>[4x]MASLARAVERLKAALERPKDEFI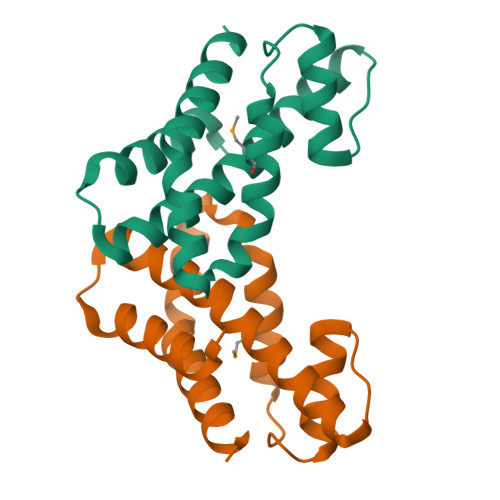RDSAIQRFEFTFELAWKTLKTFLELQGLEARSPRAAIRGAFQVGLLPEDPFWLEMLELRNLTNHTYDEALAERIYAELPKALERFQELLRRLEEPA>[2x]GPGSMVDGSDGARRVLVINSGSSSLKFQLVDPESGVAASTGIVERIGEESSPVPDHDAALRRAFDMLAGDGVDLNTAGLVAVGHRVVHGGNTFYRPTVLDDAVIARLHELSELAPLHNPPALLGIEVARRLLPGIAHVAVFDTGFFHDLPPAAATYAIDRELADRWQIRRYGFHGTSH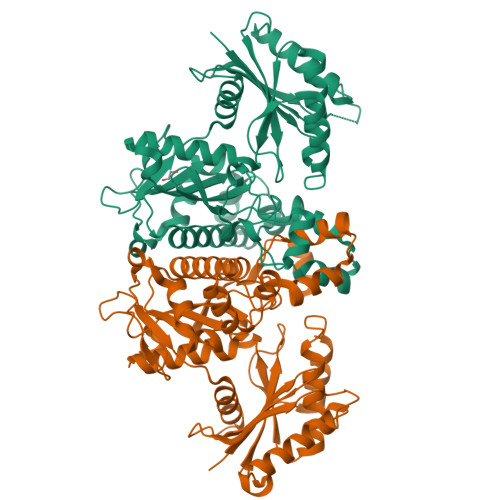RYVSEQAAAFLDRPLRGLKQIVLHLGNGCSASAIAGTRPLDTSMGLTPLEGLVMGTRSGDIDPSVVSYLCHTAGMGVDDVESMLNHRSGVVGLSGVRDFRRLRELIESGDGAAQLAYSVFTHRLRKYIGAYLAVLGHTDVISFTAGIGENDAAVRRDAVSGMEELGIVLDERRNLPGAKGARQISADDSPITVLVVPTNEELAIARDCVRVLGG> GAMGMTTYLEFIQQNEERDGVRFSWNVWPSSRLEATRMVVPVAALFTPLKERPDLPPIQYEPVLCSRTTCRAVLNPLCQVDYRAKLWACNFCYQRNQFPPSYAGISELNQPAELLPQFSSIEYVVLRGPQMPLIFLYVVDTCMEDEDLQALKESMQMSLSLLPPTALVGLITFGRMVQVHELGCEGISKSYVFRGTKDLSAKQLQEMLGLSKVPVTQATRGPQVQQPPPSNRFLQPVQKIDMNLTDLLGELQRDPWPVPQGKRPLRSSGVALSIAVGLLECTFPNTGARIMMFIGGPATQGPGMVVGDELKTPIRSWHDIDKDNAKYVKKGTKHFEALANRAATTGHVIDIYACALDQTGLLEMKCCPNLT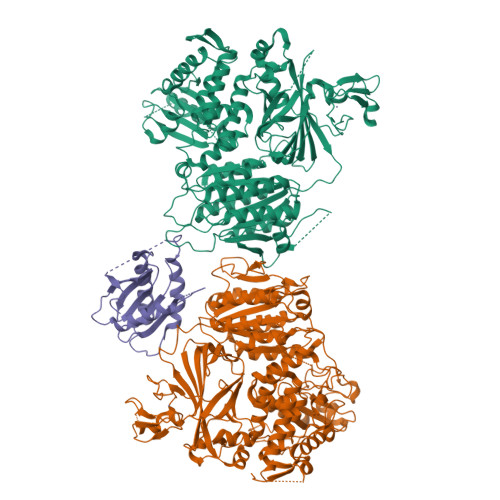GGYMVMGDSFNTSLFKQTFQRVFTKDMHGQFKMGFGGTLEIKTSREIKISGAIGPCVSLNSKGPCVSENEIGTGGTCQWKICGLSPTTTLAIYFEVVNQHNAPIPQGGRGAIQFVTQYQHSSGQRRIRVTTIARNWADAQTQIQNIAASFDQEAAAILMARLAIYRAETEEGPDVLRWLDRQLIRLCQKFGEYHKDDPSSFRFSETFSLYPQFMFHLRRSSFLQVFNNSPDESSYYRHHFMRQDLTQSLIMIQPILYAYSFSGPPEPVLLDSSSILADRILLMDTFFQILIYHGETIAQWRKSGYQDMPEYENFRHLLQAPVDDAQEILHSRFPMPRYIDTEHGGSQARFLLSKVNPSQTHNNMYAWGQESGAPILTDDVSLQVFMDHLKKLAVSSAA;> LSLQPEGLRVVNLLQERNMLPSTPLKPPVPNLHEDIQKLNCNPELFRCTLTSIPQTQALLNKAKLPLGLLLHPFKDLVQLPVVTSSTIVRCRSCRTYINPFVSFLDQRRWKCNLCYRVNDVPEEFLYNPLTRVYGEPHRRPEVQNATIEFMAPSEYMLRPPQPPVYLFVFDVSHNAVETGYLNSVCQSLLDNLDLLPGNTRTKIGFITFDSTIHFYGLQESLSQPQMLIVSDIEDVFIPMPENLLVNLNESKELVQDLLKTLPQMFTKTLETQSALGPALQAAFKLMSPTGGRMSVFQTQLPTLGVGALKPREEPNHRSSAKDIHMTPSTDFYKKLALDCSGQQVAVDLFLLSGQYSDLASLGCISRYSAGSVYYYPSYHHQHNPVQVQKLQKELQRYLTRKIGFEAVMRIRCTKGLSIHTFHGNFFVRSTDLLSLPNVNPDAGYAVQMSVEESLTDTQLVSFQSALLYTSSKGERRIRVHTLCLPVVSTLNDVFLGADVQAISGLLANMAVDRSMTASLSDARDALVNAVIDSLSAYRSSVLSNQQPGLMVPFSLRLFPLFVLALLKQKSFQTGTNARLDERIFAMCQVKNQPLVYLMLTTHPSLYRVDNLSDEGALNISDRTIPQPPILQLSVEKLSRDGAFLMDAGSVLMLWVGKNCTQNFLSQVLGVQNYASIPQPMTDLPELDTPESARIIAFISWLREQRPFFPILYVIRDESPMKANFLQNMIEDRTESALSYYEFLLHIQQQVNK;> SMVLLTMIARVADGLPLAASMQEDEQSGRDLQQYQSQAKQLFRKLNEQSPTRCTLEAGAMTFHYIIEQGVCYLVLCEAAFPKKLAFAYLEDLHSEFDEQHGKKVPTVSRPYSFIEFDTFIQKTKKLYIDSRARRNLGSINTELQDVQRIMVANIEEVLQRGEALSALDSKANNLSSLSKKYRQDAKYLNMRSTYAK Atirmociclib | 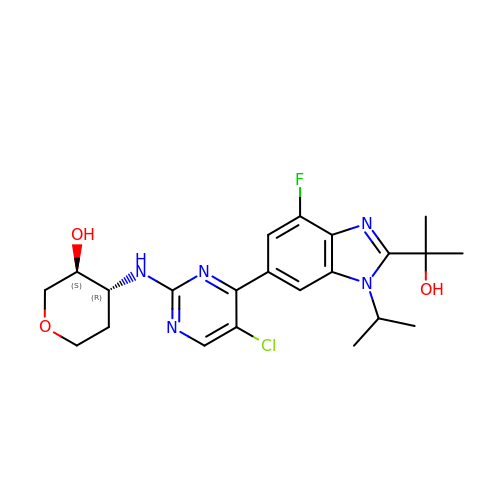C22 H27 Cl F N5 O3 | QYJLBHRAPDJOSO-NVXWUHKLSA-N> MIIDRLLQRSHSHLPILQATFGLERESLRIHQPTQRVAQTPHPKTLGSRNYHPYIQTDYSEPQLELITPIAKDSQEAIRFLKAISDVAGRSINHDEYLWPLSMPPKVREEDIQIAQLEDAFEYDYRKYLEKTYGKLIQSISGIHYNLGLGQELLTSLFELSQADNAIDFQNQLYMKLSQNFLRYRWLLTYLYGASPVAEEDFLDQKLNNPVRSLRNSHLGYVNHKDIRISYTSLKDYVNDLENAVKSGQLIAEKEFYSPVRLRGSKACRNYLEKGITYLEFRTFDLNPFSPIGITQETVDTVHLFLLALLWIDSSSHIDQDIKEANRLNDLIALSHPLEKLPNQAPVSDLVDAMQSVIQHFNLSPYYQDLLESVKRQIQSPELTVAGQLLEMIEGLSLETFGQRQGQIYHDYAWEAPYALKGYETMELSTQLLLFDVIQKGVNFEVLDEQDQFLKLWHNSHIEYVKNGNMTSKDNYIVPLAMANKVVTKKILDEKHFPTPFGDEFTDRKEALNYFSQIQDKPIVVKPKSTNFGLGISIFKTSANLASYEKAIDIAFTEDSAILVEEYIEGTEYRFFVLEGDCIAVLLRVAANVVGDGIHTISQLVKLKNQNPLRGYDHRSPLEVIELGEVEQLMLEQQGYT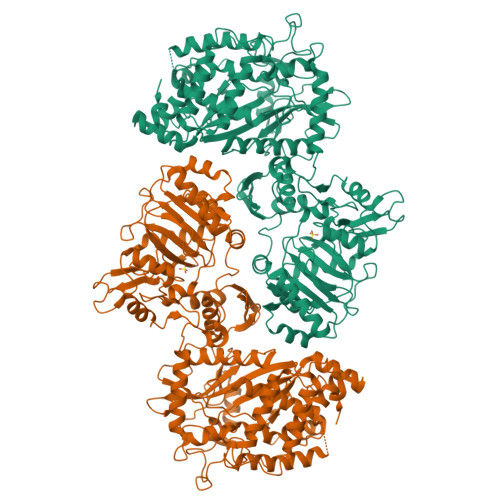VNSIPPEGTKIELRRNSNISTGGDSIDVTNTMDPTYKQLAAEMAEAMGAWVCGVDLIIPNATQAYSKDKKNATCIELNFNPLMYMHTYCQEGPGQSITPRILAKLFPEL>[2x]MIQTPLLIGFIVMALASLAIYIKGAHYGPLLGHTLIHAAVPFIAATAYLCMYLGVGNLIKVDGSVTYLARYVDWAFTTPLLLAGVVSSAYYGTRDLYGKSGYIT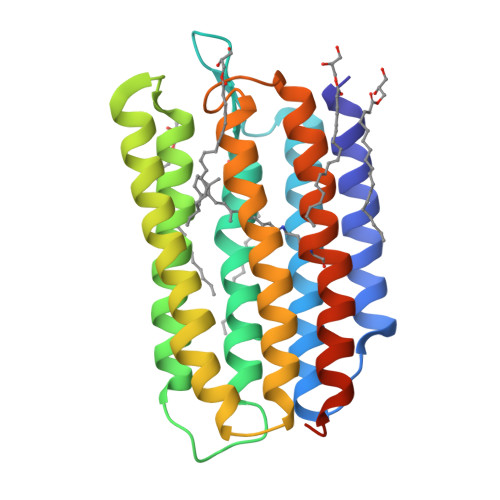AIVTLDVIMIVTGLIASLAPYGVIKWVFFAWSCAAFAGVLYLLWKPVASIASQQPGVSPAYRRNVGFLTVLWLIYPVVFAVGPEGFWAVSDATTVWVFLVLDVLAKVVYAFTSERNLRAVPVGRGYLEHHHHHH> MNKKTIRDVDVRGKRVFCRVDFNVPMEQGAITDDTRIRAALPTIRYLIEHGAKVILASHLGRPKGKVVEELRLDAVAKRLGELLERPVAKTNEAVGDEVKAAVDRLNEGDVLLLENVRFYPGEEKNDPELAKAFAELADLYVNDAFGAAHRAHASTEGIAHYLPAVAGFLMEKELEVLGKALSNPDRPFTAIIGGAKVKDKIGVIDNLLEKVDNLIIGGGLAYTFVKALGHDVGKSLLEE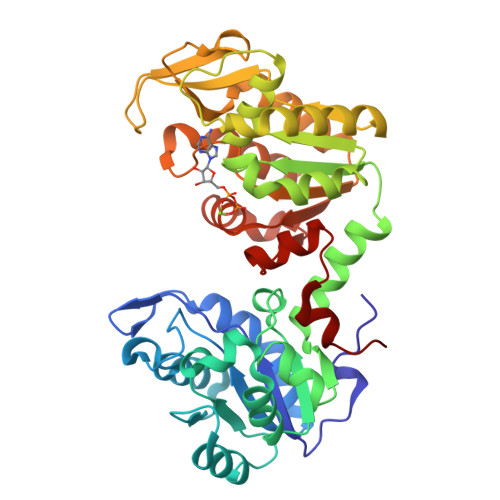DKIELAKSFMEKAKEKGVRFYMPVDVVVADRFANDANTKVVPIDAIPADWSALDIGPKTRELYRDVIRESKLVVWNGPMGVFEMDAFAHGTKAIAEALAEALDTYSVIGGGDSAAAVEKFGLADKMDHISTGGGASLEFMEGKQLPGVVALEDK>[2x]SNAMTQLTREQVL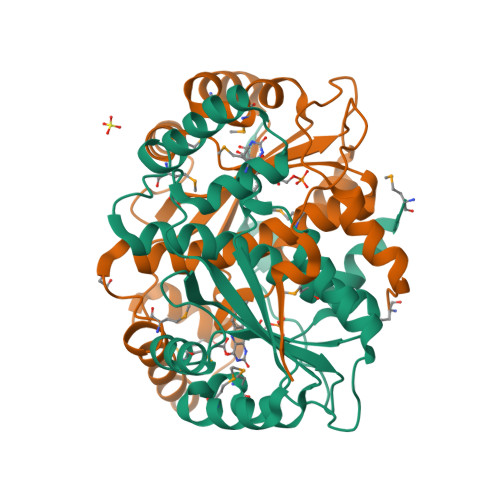ELFHQRSSTRYYDPTKKISDEDFECILECGRLSPSSVGSEPWKFLVIQNKTLREKMKPFSWGMINQLDNCSHLVVILAKKNARYDSPFFVDVMARKGLNAEQQQAALAKYKALQEEDMKLLENDRTLFDWCSKQTYIALANMLTGASALGIDSCPIEGFHYDKMNECLAEEGLFDPQEYAVSVAATFGYRSRDIAKKSRKTLDEVVKWVG> GSQSIKVKKGDTLWDLSRKYDTTISKIKSENHLRSDIIYVGQTLSINGKSTSSKSSSSSSSSSTYKVKSGDSLWKISKKYGMTINELKKLNGLKSDLLRVGQVLKLKGSTSSSSSSSSKVSSSSTSTYKVKSGDSLSKIASKYGTTVSKLKSLNGLKSDVIYVNQVLKVKGTSTSSSKPASSSSSSSSKTSS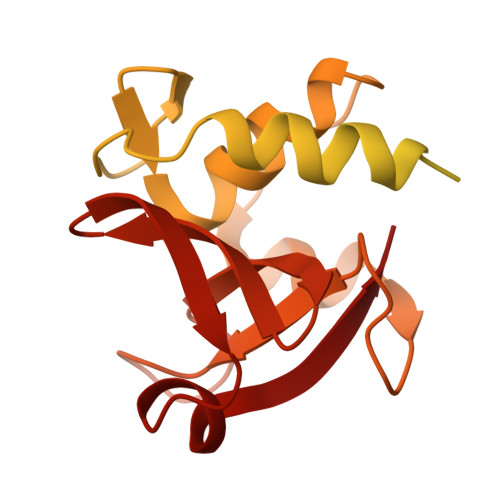TSLNVSKLVSDAKALVGTPYKWGGTTTSGFDCSGFIWYVLNKQTSVGRTSTAGYWSSMKSIASPSVGDFVFFTTYKSGPSHMGIYIGNNSFIHAGSDGVQISSLNNSYWKPRYLGAKRF> XXXXXXXXSMNGIRWIASYPKAGNTWVRCMLAAY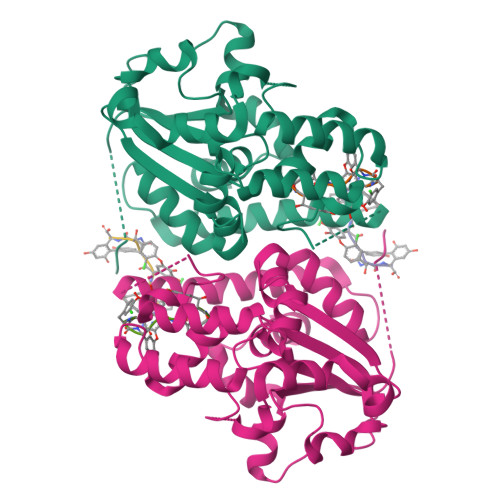ITGKAPQVWNDIDAESLTLEAMLRFGDLPPAEPMEPVLVKTHLKADVPVLGLYGEATAKVLYLVRNPRDMLLSSMRMASISRDDVEKSRDFARKFIANEGLGWNALGAGGGVGLGSWPENVRSWTESSSDRFPNADVLTMRYEDLKGDPVARFSEIVEFLDLGGPVDIEDIRRAVAASTLERMRELEKRSEQQGGGSPIRHGDARMMKGGPGGARPQFVGEGRYDQSLSFLGEDIESDYQELLHGDSGFALYAKQYGYAG>[4x]MNLPDNSIHLQLPRPVCEAIIRPVPEHRADQELSEIYRDLKATFGVPWVGVITQAVAYYRPFFAEAWRRFAPSAKTHFFERASDDIRIRSWELMGQSFVIEGQTDRLREMGYSVREIGQIRAVLDIFDYGNPKYLIFATAIKEGLLSGRTFGGAAGDARCHFPRSPICQIDPIPVMVEEHHA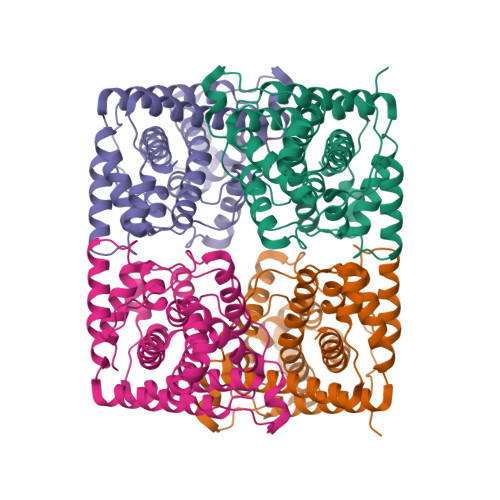GGTLSQVYADIKQTLQLPFINSDYKAMARWPSYLEQAWGALKPCIDTPAYQAGRFDINARALAALDALPTAYRMSRDDALQAGLSEAQTDELIQVISLFQWMLSGLVLNVTHFKQQALK> GAMAETVFKQNHAASGFLAGRYDAQAMS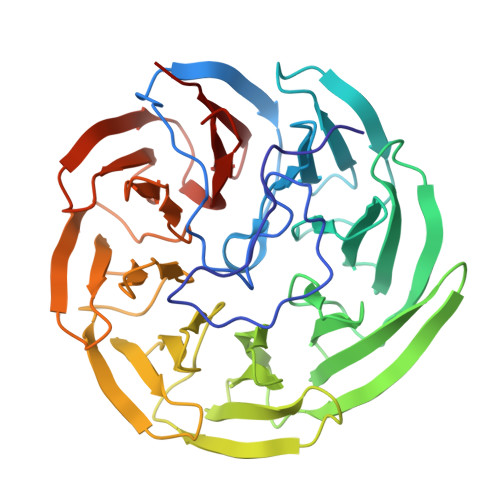PTMFNWSRESRFTSTADGALKWEKNVPATPQNGAGAAVDGDGTVFIQSKDGKLTAYHPDGTVKWVTENLGTTYTLTPVLGTNGVIYLPSHDKKLYFIDKETGNILWSVPLSGAPSSDAAIGPDGTLYVSTLDNYIYAIKPTSPGTATQKWKFKTNGVVGSAPVLASNGTLYTATYNNIFYAINSGTGQVKWSKTTSNGFKGYPVIDRDGTVYAGNQDGNLYAYTSTGAVKWTFPLNGFSSSSLAIDHNGNVYIGSGSGELFSISKTGNMNWSFYTDGPVRTAPLIDADGNVYFGSDDKNVYAVDADGNEKWRYQTDSNVISSPVLAEDGTLYVGTYTKLLAFGAK> AAQTNAPWGLARISSTSPGTSTYYYDESAGQGSCVYVIDTGIEASHPEFEGRAQMVKTYYYSSRDGNGHGTHCAGTVGSRTYGVAKKTQLFGVKVLDDNGSGQYSTIIAGMDFVASDKNNRNCPKGVVASLSLGGGYSSSVNSAAARL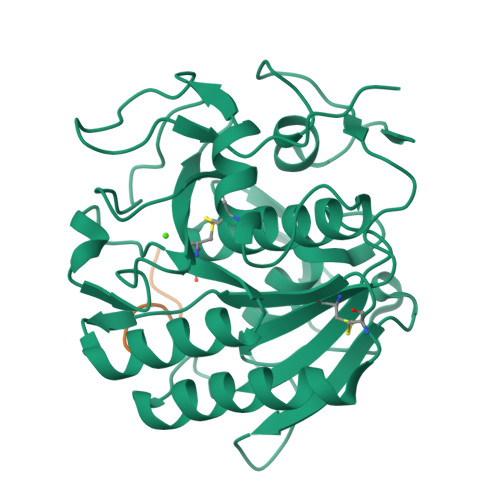QSSGVMVAVAAGNNNADARNYSPASEPSVCTVGASDRYDRRSSFSNYGSVLDIFGPGTDILSTWIGGSTRSISGTSMATPHVAGLAAYLMTLGKTTAASACRYIADTANKGDLSNIPFGTVNLLAYNNYQA;> GDEQGENK> MEGGKLQSTFVFEEIGRRLKDIGPEVVKKVNAVFEWHITKGGNIGAK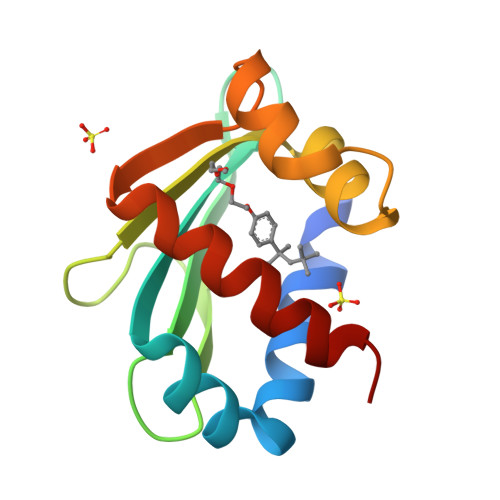WTIDLKSGSGKVYQGPAKGAADTTIILSDEDFMEVVLGKLDPQKAFFSGRLKARGNIMLSQKLQMILKDYAKL> MTKWNYGVFFLNFYHVGQQEPSLTMSNALETLRIIDEDTSIYDVVAFSEHHIDKSYNDETKLAPFVSLGKQIHVLATSPETVVKAAKYGMPLLFKWDDSQQKRIELLNHYQAAAAKFNVDIANVRHRLMLFVNVNDNPTQAKAELSIYLE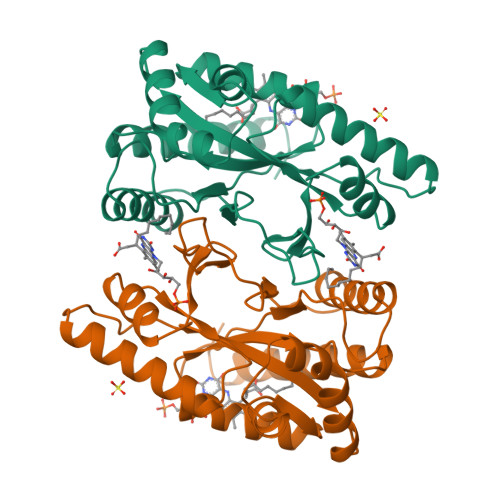DYLSYTQAETSIDEIINSNAAGNFDTCLHHVAEMAQGLNNKVDFLFCFESMKDQENKKSLMINFDKRVINYRKEHNLN>MKTQIINGVSLPNIPWQDKPADCKDVIWRYDANPIIPRDQLPTSNSIFNSAVVPYESEKGKFAGVFRVDDKCRNMELHAGFSKDGIHWDINPDRIVFEQAEKSTEEVNQWGYGYDPRVCFIEDRFWVTWCNAYGWKPTIGVAYTFDFKTFYQCENAFLPFNRNGVLFPRKINGKYVMFSRPSDSGHTPFGDMFISQSPDMKYWGEHRHVMGPLRAWESKKIGAGPIPIETSEGWLCFYHGVLESCNGFVYSFSACILDKDEPWKVKYRCAEYLLSPQ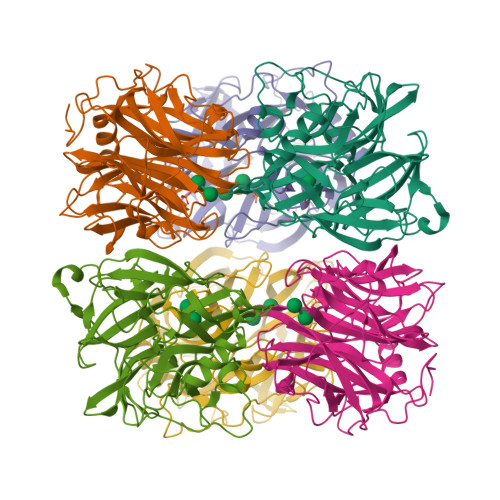KIYECVGDVQNVTFPCATLVDADTGRIAIYYGCADTCVSMAFTTVDDVVDYVKSHSSV[6x]> SRLNRESVIDAALELLNETGIDGLTTRKLAQKLGIEQPTLYWHVKNKRALLDALAVEILARHHDYSLPAAGESWQSFLRNNAMSFRRALLRYRDGAKVHLGTRPDEKQYDTVETQLRFMTENGFSLRDGLYAISAVSHFTLGAV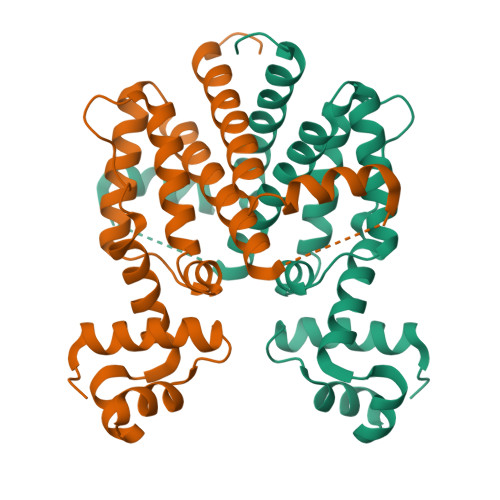LEQQEHTAALTDRPAAPDENLPPLLREALQIMDSDDGEQAFLHGLESLIRGFEVQLTALLQIV>PASEEEFQFLRCQQCQAEAKCPKLLPCLHTLCSGCLEASGMQCPICQAPWPLGADTPALDNVFFESLQRRLSVYRQIVDAQAVCTRCKESADFWCFECEQLLCAKCFEAHQWFLKHEARPLAELRNQSVREFLDGTRKTNNIFCSNPNHRTPTLTSIYCRGCSKPLCCSCALLDSSHSELKCDISAEIQQRQEELDAMTQALQEQDSAFGA[2x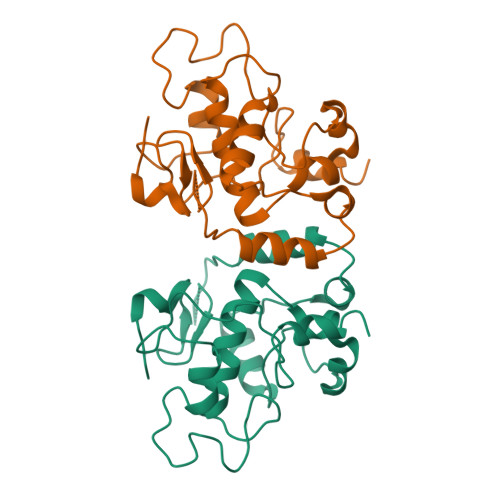]>DSSDEASVSPIADNEREAVTLLLGYLEDKDQLDFYSGGPLKALTTLVYSDNLNLQRSAALAFAEITEKYVRQVSREVLEPILILLQSQDPQIQVAACAALGNLAVNNENKLLIVEMGGLEPLINQMMGDNVEVQCNAVGCITNLATRDDNKHKIATSGALIPLTKLAKSKHIRVQRNATGALLNMTHSEENRKELVNAGAVPVLVSLLSSTDPDVQYYCTTALSNIAVDEANRKKLAQTEPRLVSKLVSLMDSPSSRVKCQATLALRNLASDTSYQLEIVRA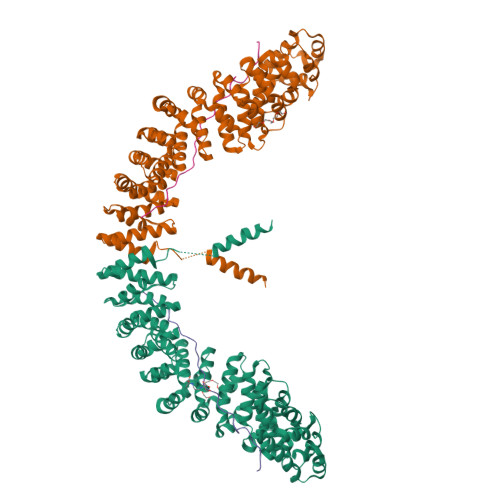GGLPHLVKLIQSDSIPLVLASVACIRNISIHPLNEGLIVDAGFLKPLVRLLDYKDSEEIQCHAVSTLRNLAASSEKNRKEFFESGAVEKCKELALDSPVSVQSEISACFAILALADVSKLDLLEANILDALIPMTFSQNQEVSGNAAAALANLCSRVNNYTKIIEAWDRPNEGIRGFLIRFLKSDYATFEHIALWTILQLLESHNDKVEDLVKNDDDIINGVRK[2x];>[2x]NREKDCSSSSEVESQSKCRKESTAEPDSLSRDTRTTSSLKSSTSFPISFKGSIDLKSLNQPSSLLHIQVSPTKSSNLDAQVNTEQAYSQPFRY> MGGLLFSSLQHCQQGFVISNELRQQQSELTSTWDLMLQTRINLSRSAARMMMDASNQQ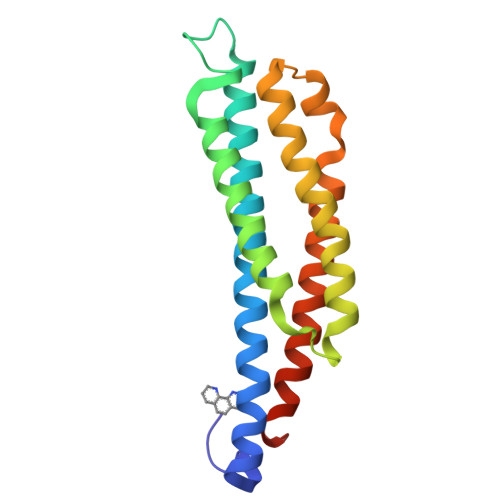SSAKTDLLQNAKTTLAQAAAHYANFKNMTPLPAMAEASANVDEKYQRYQAALAELIQFLDNGNMDAYFAQPTQGMQNALGEALGNYARVSENLYRQTFDQSAHDYR>[2x]LTLWTTLDPSPNCKIDIEKDSKLTLVLTKCGSQILANVSLIIVNGKFKILNNKTDPSLPKSFNIKLLFDQNGVLLENSNIEKQYLNFRSGDSILPEPYKNAIGFMPNLLAYAKATTDQSKIYARNTIYGNIYLDNQPYNPVVIKITFNNEADSAYSITFNYSWTKDYDNIPFDSTSFTFSYIAQE

Species D (HAdV-D) are the most diverse species and cause both gastrointestinal tract infections and epidemic keratoconjunctivitis (EKC). Each protein forms key interactions to promote cell infection, with the terminal domain of the fiber, the fiber knob protein, interacting with the viruses’ primary cell entry receptor. The adenovirus fiber knob protein is known to have a highly conserved trimeric structure. Sialic acid (SA) usage has been proposed as a major mechanism of cell infection for EKC causing HAdV-D. Here, we provide apo state crystal structures for fiber knob proteins of 7 previously undetermined HAdV-D, and provide crystal structures of HAdV-D25, HAdV-D29 and HAdV-D53 knob proteins bound to SA.

To evaluate the potential for these recombinant fiber knob proteins to bind cellular sialic acid residues, crystals of the fiber-knob proteins were also soaked with sialic acid prior to data collection. This resulted in four structures of HAdV-D25, D29, D30 and D53 in complex with sialic acid also shown in [Fig fig1]. The conformation of the bound sialic acid was found to be a mixture of the *a* and ß anomers, freely exchangeable in solution and minimal protein side chain adjustment was required to accommodate either conformation. Soaking in sialic acid containing solutions reduced resolution slightly. [Fig fig2] panels A-E depicts these pockets in fiber knob proteins of HAdV-D25, D29, D30 and D53, where sialic acid is coloured according to structure and the residues contacting sialic acid are shown in green. Y314 and K349 (according to HAdV-D26 sequence) are conserved across all sequences, while the remaining residues are similar, suggesting the existence of a common sialic acid binding pocket across all species fiber knob proteins. Whilst the threonine was not found to be universally conserved ([Fig fig2]), the other species D adenoviruses had similar sized residues which generally made interactions with sialic acid in HAdV-D29, D30 and D53 ([Fig fig2] and [Fig fig2]). Pseudotyped viruses comprising an HAdV-C5 core viral vector psedutoyped with the fiber knob proteins of several HAdV-D of interest (D26, D15, D24, D29 and D53) were generated expressing a luciferase transgene under the control of a ubiquitous CMV IE promoter for measuring transduction following cell treatment with and without neuraminidase treatment. Non-significant changes in transduction were observed when cells were transduced with viruses with the fiber-knob proteins of HAdV-D15, D24 and D29 ([Fig fig3]). There was an overall trend in reduction, although in BT-20 cells there was a small, non-significant, increase in transduction of HAdV-D29 fiber-knob protein virus following treatment with neuraminidase.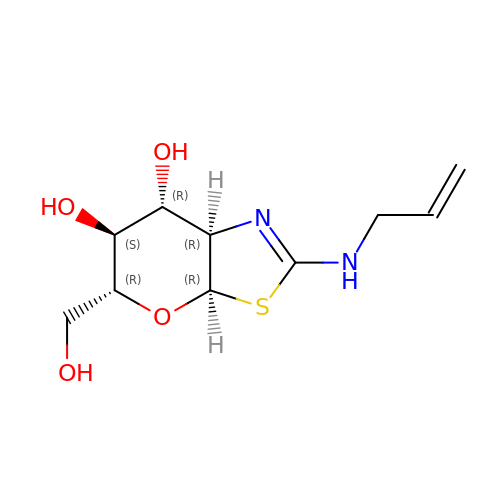(3~{a}~{R},5~{R},6~{S},7~{R},7~{a}~{R})-5-(hydroxymethyl)-2-(prop-2-enylamino)-5,6,7,7~{a}-tetrahydro-3~{a}~{H}-pyrano[3,2-d][1,3]thiazole-6,7-diol | C10 H16 N2 O4 S | RFYRJQYZBZAHNY-JGKVKWKGSA-N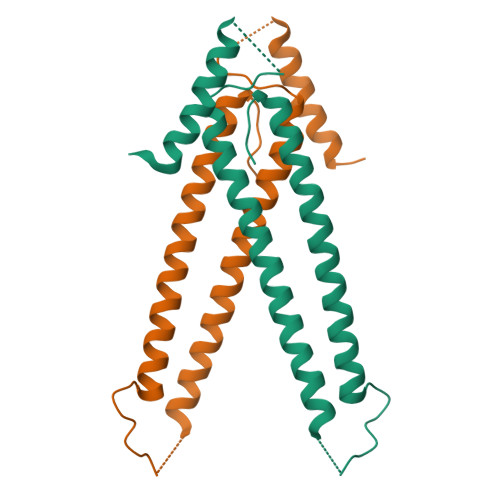>GVVNHTEMENLRVQLEEAERRLEANSNGSQAPLALQPLLRRTCENEMAFLEKQRQDCFKEMKEAIEMVDRLQKKQGSVLSSLKLATGAASTSDQVDSKIFALKSRMEKIHTLTRETQERWLQIESLCGFPLLYLNE[2x]>[2x]MQVPILEKFCFTPHTEEGCLSERAALQEELQLCKGLVQALQTKVTQQGLKMVVPGLDGAQIPRDPSQQELPRLLSAACRLQLNGNLQLE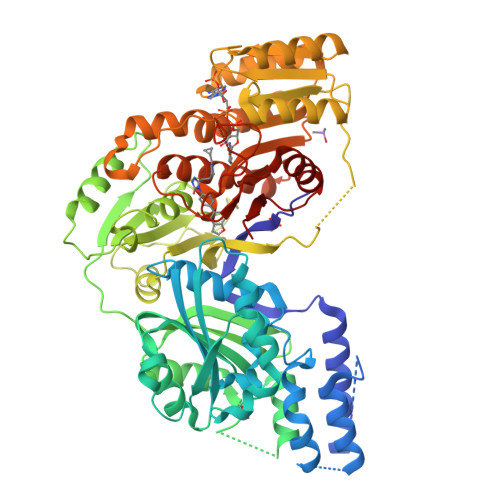LAQVLAQERPKLPEDPLLSGLLDSPALKACLDTAVENMPSLKMKVVEVLAGHGHLYSRIPGLLSPHPLLQLSYTATDRHPQALEAAQAELQQHDVAQGQWDPADPAPSALGSADLLVCNCAVAALGDPASALSNMVAALREGGFLLLHTLLRGHPLGDIVAFLTSTEPQYGQGILSQDAWESLFSRVSLRLVGLKKSFYGSTLFLCRRPTPQDSPIFLPVDDTSFRWVESLKGILADEDSARPVWLKAINCATSGVVGLVNCLRREPGGNRLRCVLLSNLSSTSHVPEVDPGSAELQKVLQGDLVMNVYRDGAWGAFRHFLLEEDKGSKTFCPAHKSYIIAGGLGGFGLELAQWLIQRGVQKLVLTSRSGIRTGYQAKQVRRWRRQGVQVQVSTSNISSLEGARGLIAEAAQLGPVGGVFNLAVVLRDGLLENQTPEFFQDVCKPKYSGTLNLDRVTREACPELDYFVVFSSVSCGRGNAGQSNYGFANSAMERICEKRRHEGLPGLAVQWGAIGDVGILVETMSTNDTIVSGTLPQRMASCLEVLDLFLNQPHMVLSSFVLAEKHHHHHH>ANNRAEVDTLSPAQAAELKPMPQSWRGVLPCADCEGIETSLFLEKDGTWVMNERYLGAREEPSSFASYGTWARTADKLVLTDSKGEKSYYRAKGDALEMLDREGNPIESQFNYTLEAAQSSLPMTPMTLRGMYFYMADAATFTDCATGKRFMVANNAELERSYLAARGHSEKPVLLSVE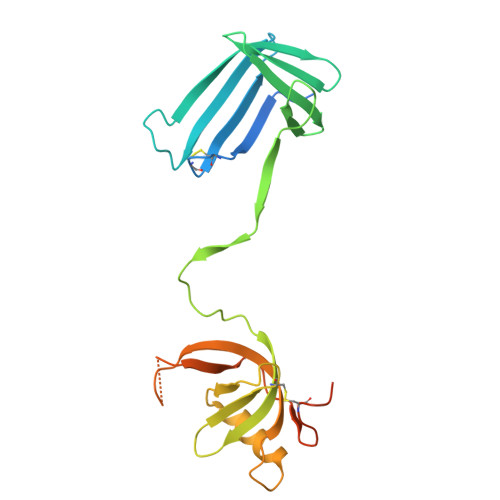GHFTLEGNPDTGAPTKVLAPDTAGKFYPNQDCSSLGQMASMTGGQQMGHHHHHH[2x]>[8x]ALESLRGNADLAYILSMEPCGHCLIINNVNFCRESGLRTRTGSNIDCEKLRRRFSSLHFMVEVKGDLTAKKMVLALLELARQDHGALDCCVVVILSHGCQASHLQFPGAVYGTDGCPVSVEKIVNIFNGTSCPSLGGKPKLFFIQACGGEQKDHGFEVASTSPEDESPGSNPEPDATPFQEGLRTFDQLDAISSLPTPSDIFVSYSTFPGFVS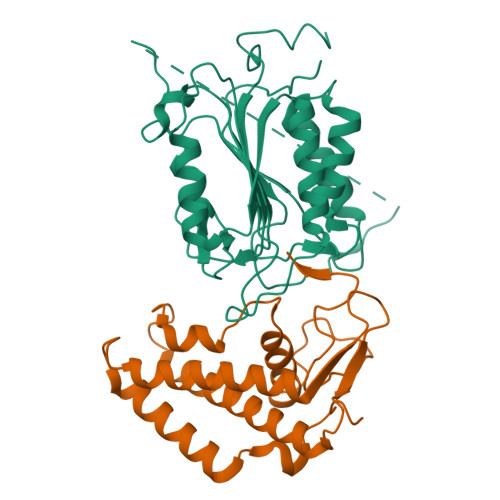WRDPKSGSWYVETLDDIFEQWAHSEDLQSLLLRVANAVSVKGIYKQMPGCFNFLRKKLFFKTS;>TPESVSELNHNHFLSPELQDKLDVMVSIYSCARNNNELEEIFQELSAFVSGLMDKRNSVFEVRNENTDEVVGALRAGMTIEDRDSYIRDLFFLHSLKVKIEESRQGKEDSKCKVYNLLCPHHSSELYGDLRAMKCLVEGCSDDFNPFDIIRVPDLTYNKGSLQCG[8x]SulE, an esterase, which detoxifies a variety of sulfonylurea herbicides through de-esterification, provides an attractive approach to remove environmental sulfonylurea herbicides and develop herbicide-tolerant crops. SulE catalyzes the de-esterification of a variety of sulfonylurea herbicides, such as MM, BM, SM, TM, TrM, EM, and CE, to the corresponding herbicidal-inactive parent acid. The structures show that SulE is a dimer with a lid loop in a domain-swapped β-hairpin covering the active site from the opposing monomer. SulE shows a similar catalytic triad consisting of Ser209, His333, and Glu232 at its active site.

SulE was overexpressed in E. coli BL21 (DE3), purified, and crystallized in a space group P21. The asymmetric unit contains two monomers. SulE is a homodimer, consistent with its oligomerization state in solution as determined by gel filtration chromatography. For each monomer, residues 12–360 are clearly defined based on the electron densities. The overall structure of SulE monomer contains a catalytic domain (residues 12–27, 55–112, and 185-360), a cap domain (residues 113–184) and a protruding β hairpin (residues 28–54). The catalytic domain is a typical α/β hydrolase fold, with eight β-strands (β1 to β8), six α-helices (α1 to α6) and two 310-helices (η1 and η2). The cap domain (residues 113–184) is inserted in the loop connecting β4 and α2 and is composed of two α-helices (αCAP1 and αCAP2). Particularly, a β hairpin, which contains a lid loop (residues 31–51) between β9 and β10, is far away from the core region in each subunit, but cover the cap domain and close to the active center of another subunit in the dimer structure. His333 Nε2 is hydrogen bonded to Ser209 Oγ at a distance of 2.79 Å, and is responsible for the activation of the nucleophile Ser209. Glu232 Oδ2 is strongly hydrogen bonded to His333 Nδ1 at a distance of 2.64 Å to correctly position the imidazole ring of His333 for catalysis.

>[2x]METDNVELAQSKRKVVLAEQGSFYIGGRTVTGPGKFDPSKPVIPYSNEGATFYINQMYVNFQAPVRPRGLPLVFWHGGGLTGHIWESTPDGRPGFQTLFVQDRHTVYTIDQPGRGRGNIPTFNGPFGQLEEESIVNTVTGNSSKEGAWVRDRLGPAPGQFFENSQFPRGYEDNYFKEMGFSPSISSDEIVDAVVKLVTHIGPCVLVTHSASGVLGMRVATHAKNVRGIVAYEPATSIFPKGKVPEIPPLADKKSQIFPPFEIQESYFKKLAKIPIQFVFGDNIPKNPKSAYWFLDWWRVTRYAHSLSLEAINKLGGQASLLDLPTAGLRGNTHFPFTDRNNVQVASLLSDFLGKHGLDQNESLEHHHHHH> GAMGSGTARPGRSKVFNPYTEFPEFSRRLLKDLEKMFKTYDAGRDGFIDLMELKLMMEKLGAPQTHLGLKSMIKEVDEDFDGKLSFREFLLIFHKAAAGELQEDSGLLALAKFSEIDVALEGVRGAKNFFEAKAQA

The EF-hand domain-containing protein 1 (EFhd1), a homologous protein of EFhd2, is localized in the mitochondria. Unlike EFhd2 and AIF-1, EFhd1 is localized in the mitochondria and may regulate mitochondrial energy metabolism. Here, we report the crystal structure of the core domain of mouse EFhd1 (CDEFhd1, residues 79–180) in a Ca2+-bound state, comprising a proline-rich (PR) region, two EF-hand motifs, a ligand mimic helix (LM-helix), and a C-terminal linker. In addition, we identified Ca2+-independent α- and β-actin-binding and Ca2+-dependent β-actin-bundling activities of EFhd1, indicating that EFhd1 might be involved in the Ca2+-dependent regulation of mitochondrial morphology via interactions with β-actin.

We determined the crystal structure of the core domain of mouse EFhd1 (CDEFhd1, residues 79–180) at a resolution of 2.07 Å and refined to Rwork = 20.9 (%) and Rfree = 22.9 (%). We initially attempted to crystallize the EFhd1 ΔNTD (residues 69–240) construct, but only the core domain was crystallized due to proteolytic degradation. The CDEFhd1 structure comprised two EF-hand motifs (residues 91–162), an LM-helix (residues 169–176), a C-terminus of the PR region (residues 79–89) at the N-terminus, and a C-terminal linker (residues 177–180). Within the structure, Ca2+ ions were coordinated in each of the two EF-hand motifs of CDEFhd1. Collectively, EF-hand 1 and EF-hand 2 of CDEFhd1 had a distorted or general geometry for Ca2+ coordination, respectively. Collectively, CDEFhd1 formed a compact and rigid domain structure through these intramolecular interactions. Although the sequence conservation was limited to the EF-hand motifs in AIF-1, the overall structures of these proteins for Ca2+-bound states were relatively well-superimposed (RMSD of CDEFhd1 and CDEFhd2 = 0.403 Å for 85 Cα atoms, RMSD of CDEFhd1 and AIF-1 = 2.089 Å for 63 Cα atoms). Collectively, the overall structure of CDEFhd1 was similar to that of CDEFhd2 and AIF-1, but the hydrophobic interaction network between the LM-helix and hydrophobic groove of EF-hands in CDEFhd1 was similar to that of CDEFhd2, but not AIF-1. We identified two Zn2+-mediated interactions between one CDEFhd1 (MolA) and other symmetry-mate molecules (MolB and MolC). Zn1 was coordinated by H129 (MolB), K133 (MolB), H157 (MolA), and E163 (MolA), and Zn2 was coordinated by D142 (MolA), D144 (MolA), a water molecule, and E166 (MolC).> GPLGSPEFMALAVAPWGRQWEEARALGRAVRMLQRLEEQCVDPRLSVSPPSLR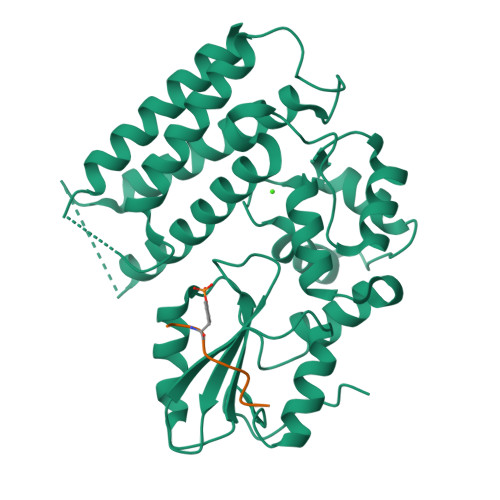DLLPRTAQLLREVAHSRRAAGGGGPGGPGGSGDFLLIYLANLEAKSRQVAALLPPRGRRSANDELFRAGSRLRRQLAKLAIIFSHMHAELHALFPGGKYCGHMYQLTKAPAHTFWRESCGARCVLPWAEFESLLGTCHPVEPGCTALALRTTIDLTCSGHVSIFEFDVFTRLFQPWPTLLKNWQLLAVNHPGYMAFLTYDEVQERLQACRDKPGSYIFRPSCTRLGQWAIGYVSSDGSILQTIPANKPLSQVLLEGQKDGFYLYPDGKTHNPDLTELG;> EDSFLQRYSSDPT>[2x]PGSGPVFVQEPSHVMFPLDSEEKKVKLSCEVKGNPKPHIRWKLNGTD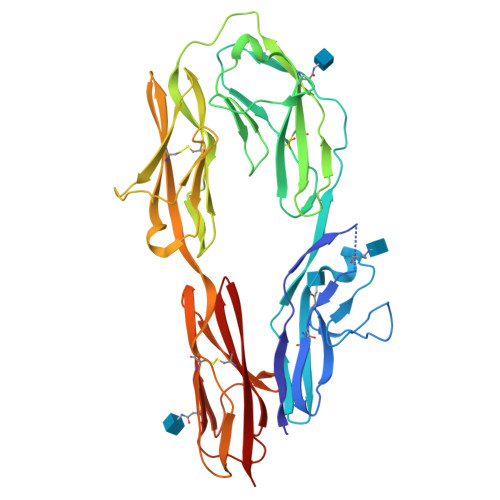VDIGMDFRYSVVDGSLLINNPNKTQDAGTYQCIATNSFGTIVSREAKLQFAYLENFKTRTRSTVSVRRGQGMVLLCGPPPHSGELSYAWIFNEYPSYQDNRRFVSQETGNLYIAKVEKSDVGNYTCVVTNTVTNHKVLGPPTPLILRNDGVMGEYEPKIEVQFPETVPAEKGTTVKLECFALGNPVPTILWRRADGKPIARKARRHKSNGILEIPNFQQEDAGSYECVAENSRGKNVAKGQLTFYAQPNWVQIINDIHVAMEESVFWECKANGRPKPTYRWLKNGDPLLTRDRIQIEQGTLNITIVNLSDAGMYQCVAENKHGVIFSSAELSVIAE>[2x]MDHLPIF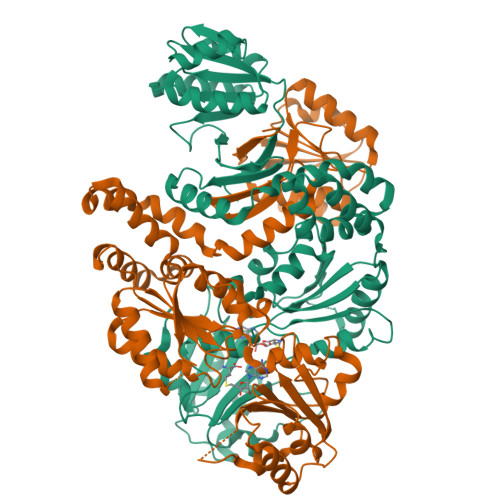CQLRDRDCLIVGGGDVAERKARLLLEAGARLTVNALTFIPQFTVWANEGMLTLVEGPFDETLLDSCWLAIAATDDDTVNQRVSDAAESRRIFCNVVDAPKAASFIMPSIIDRSPLMVAVSAGGTSHVLARLLREKLESLLPQHLGQVARYAGQLRARVKKQFATMGERRRFWEKFFVNDRLAQSLANADEKAVNATTERLFSEPLDHRGEVVLVGAGPGDAGLLTLKGLQQIQQADIVVYDRLVSDDIMNLVRRDADRVFVGKRAGYHCVPQEEINQILLREAQKGKRVVRLKGGDPFIFGRGGEELETLCHAGIPFSVVPGITAASGCSAYSGIPLTHRDYAQSVRLVTGHLKTGGELDWENLAAEKQTLVFYMGLNQAATIQEKLIAFGMQADMPVALVENGTSVKQRVVHGVLTQLGELAQQVESPALIIVGRVVALRDKLNWFSNH>[2x]SAVKAARYGKDNVRVYKVHKDEKTGVQTVYEMTVCVLLEGEIETSYTKADNSVIVATDSIKNTIYITAKQNPVTPPELFGSILGTHFIEKYNHIHAAHVNIVCHRWTRMDIDGKPHPHSFIRDSEEKRNVQVDVVEGKGIDIKSSLSGLTVLKST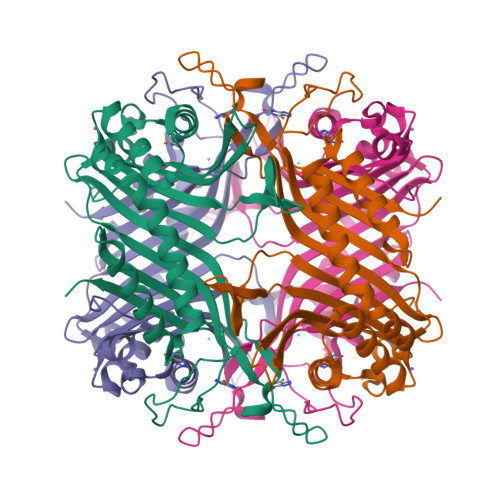NSQFWGFLRDEYTTLKETWDRILSTDVDATWQWKNFSGLQEVRSHVPKFDATWATAREVTLKTFAEDNSASVQATMYKMAEQILARQQLIETVEYSLPNKHYFEIDLSWHKGLQNTGKNAEVFAPQSDPNGLIKCTVGRS> MAGAIIENMSTKKLCIVGGILLVFQIIAFLVGGLIAPGPTTAVSYMSVKCVDARKNHHKTKWFVPWGPNHCDKIRDIEEAIPREIEANDIVFSVHIPLPHMEMSPWFQFMLFILQLDIAFKLNNQIRENAEVSMDVSLAYRDDAFAEWTEMAHERVPRKLKCTFTSPKTPEHEGRYYECDVLPFMEIGSVAHKFYLLNIRLPVNEKKKINVGIGEIKDIRLVGIHQNGGFTKVWFAMKTFLTPSIFIIMVWYWRRITMMSRPPVLLEKVIFALGISMTFINIPVEWFSIGFDWTWMLLFGDIRQGIFYAMLLSFWIIFCGEHMMDQHERNHIAGYWKQVGPIAVGSFCLFIFDMCERGVQLTNPFYSIWTTDIGTELAMAFIIVAGICLCLYFLFLCFMVFQVFRNISGKQSSLPAMSKVRRLHYEGLIFRFKFLMLITLACAAMTVIFFIVSQVTEGHWKWGGVTVQVNSAFFTGIYGMWNLYVFALMFLYAPSHKNYGEDQSNGDLGVHSGEELQLTTTITHVDGPTEIYKLTRKEAQEAENLYFQSHHHHHHHHHHDYKDDDDK;> MGNLFMLWAALGICCAAFSASAWSVNNFLITGPKAYLTYTTSVALGAQSGIEECKFQFAWERWNCPENALQLSTHNRLRSATRETSFIHAISSAGVMYIITKNC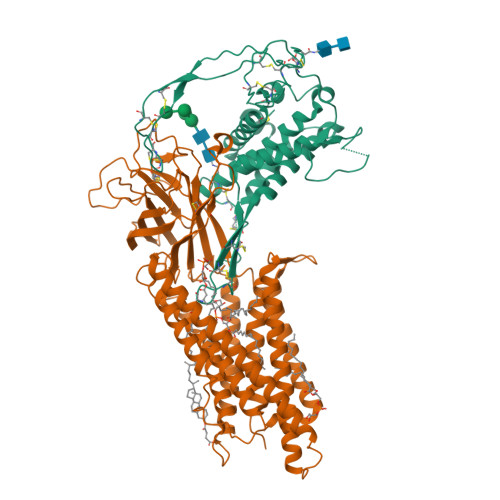SMGDFENCGCDGSNNGKTGGHGWIWGGCSDNVEFGERISKLFVDSLEKGKDARALMNLHNNRAGRLAVRATMKRTCKCHGISGSCSIQTCWLQLAEFREMGDYLKAKYDQALKIEMDKRQLRAGNSAEGHWVPAEAFLPSAEAELIFLEESPDYCTCNSSLGIYGTEGRECLQNSHNTSRWERRSCGRLCTECGLQVEERKTEVISSCNCKFQWCCTVKCDQCRHVVSKYYCARSPGSAQSLGKGSAGGWSHPQFEK>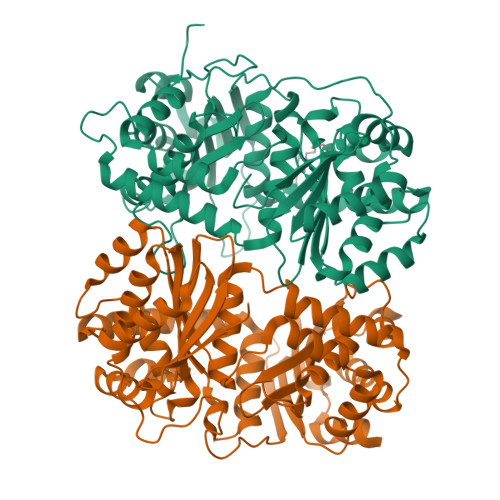[4x]ARTDNFKLSSLANGLKVATSNTPGHFSALGLYIDAGSRFEGRNLKGCTHILDRLAFKSTEHVEGRAMAETLELLGGNYQCTSSRENLMYQASVFNQDVGKMLQLMSETVRFPKITEQELQEQKLSAEYEIDEVWMKPELVLPELLHTAAYSGETLGSPLICPRGLIPSISKYYLLDYRNKFYTPENTVAAFVGVPHEKALELTGKYLGDWQSTHPPITKKVAQYTGGESCIPPAPVFGNLPELFHIQIGFEGLPIDHPDIYALATLQTLLGGGGSFSAGGPGKGMYSRLYTHVLNQYYFVENCVAFNHSYSDSGIFGISLSCIPQAAPQAVEVIAQQMYNTFANKDLRLTEDEVSRAKNQLKSSLLMNLESKLVELEDMGRQVLMHGRKIPVNEMISKIEDLKPDDISRVAEMIFTGNVNNAGNGKGRATVVMQGDRGSFGDVENVLKAYGLGNSSSSKNDSPKKKGWFHHHHHH;>ASQIPGTRTSKLPNGLTIATEYIPNTSSATVGIFVDAGSRAENVKNNGTAHFLEHLAFKGTQNRPQQGIELEIENIGSHLNAYTSRENTVYYAKSLQEDIPKAVDILSDILTKSVLDNSAIERERDVIIRESEEVDKMYDEVVFDHLHEITYKDQPLGRTILGPIKNIKSITRTDLKDYITKNYKGDRMVLAGAGAVDHEKLVQYAQKYFGHVPKSESPVPLGSPRGPLPVFCRGERFIKENTLPTTHIAIALEGVSWSAPDYFVALATQAIVGNWDRAIGTGTNSPSPLAVAASQNGSLANSYMSFSTSYADSGLWGMYIVTDSNEHNVRLIVNEILKEWKRIKSGKISDAEVNRAKAQLKAALLLSLDGSTAIVEDIGRQVVTTGKRLSPEEVFEQVDKITKDDIIMWANYRLQNKPVSMVALGNTSTVPNVSYIEEKLNQ[4x]> ACACGTGGACGACTGCGAG;> TGCTCGCAGTCGTGGTC;> CAGAC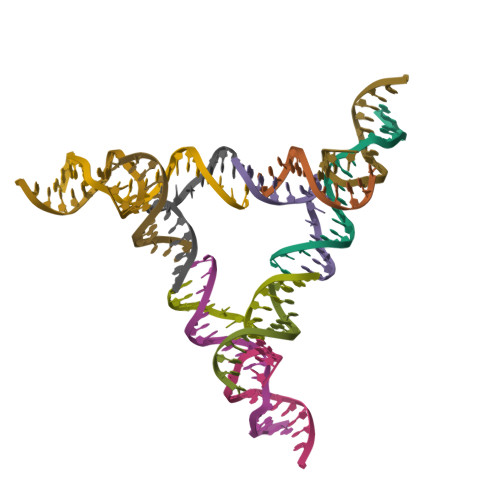CTGACTC;> TGAGTCACCACGTG>[3x]MAAQATAETPAGELPVIDAVTTHAPEVPPAIDRDYPAKVRVKMETVEKTMKMDDGVEYRYWTFDGDVPGRMIRVREGDTVEVEFSNNPSSTVPHNVDFHAATGQGGGAAATFTAPGRTSTFSFKALQPGLYIYHCAVAPVGMHIANGMYGLILVEPKEGLPKVDKEFYIVQGDFYTKGKKGA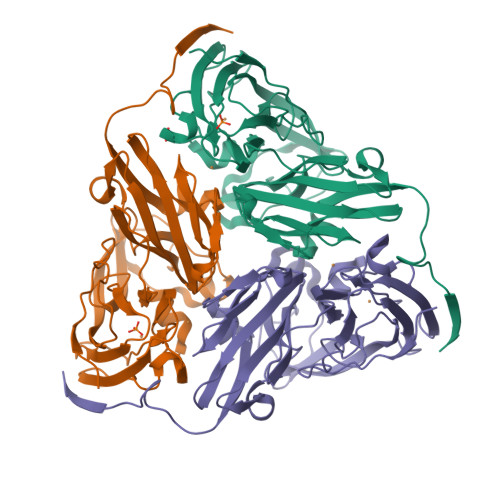QGLQPFDMDKAVAEQPEYVVFNGHVGAIAGDNALKAKAGETVRMYVGNGGPNLVSSFHVIGEIFDKVYVEGGKLINENVQSTIVPAGGSAIVEFKVDIPGNYTLVDHSIFRAFNKGALGQLKVEGAENPEIMTQKLSDTAYAVPRGSLEHHHHHH S-MERCAPTOCYSTEINE | C3 H7 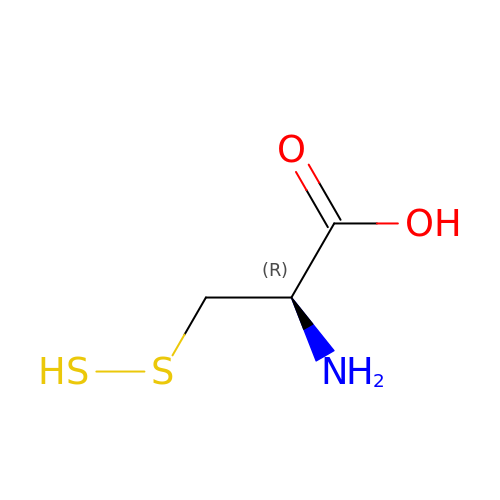N O2 S2 | XBKONSCREBSMCS-REOHCLBHSA-N DENDRON-D3 | C69 H77 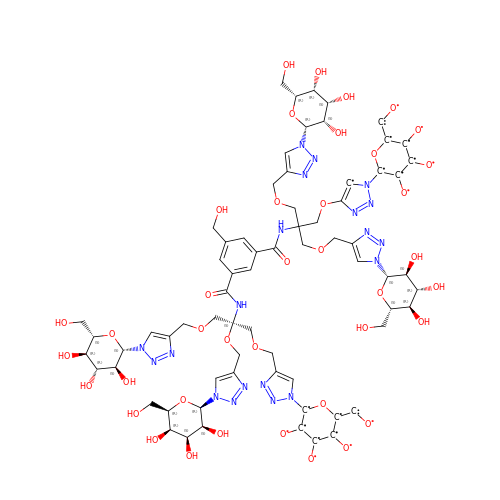N20 O39 | UIPCUAWHWTZJAS-NIRXFCQJSA-N> MKKGHHHHHHGSERTGTQPLGVQGLTEEQRMMIRELMDAQMKTFDTTFS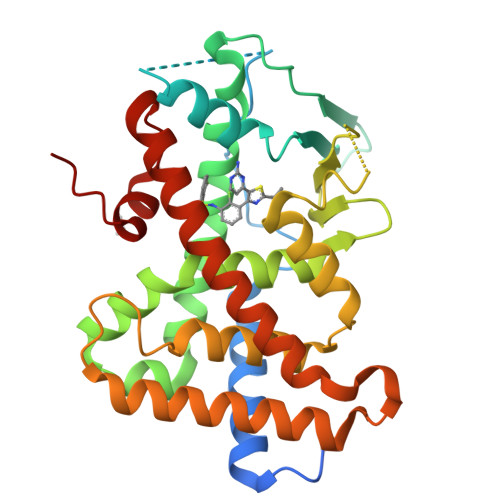HFKNFRLPGVLSSGCELPESLQAPREEAAKWSQVRKDLCSLKVSLQLRGEDGSVWNYKPPADSGGKEIFSLLPHMADMSTYMFKGIISFAKVISYFRDLPIEDQISLLKGAAFELCQLRFNTVFNAETGTWECGRLSYCLEDTAGGFQQLLLEPMLKFHYMLKKLQLHEEEYVLMQAISLFSPDRPGVLQHRVVDQLQEQFAITLKSYIECNRPQPAHRFLFLKIMAMLTELRSINAQHTQRLLRIQDIHPFATPLMQELFGITGS> MANPYERGPNPTDALLEARSGPFSVSEERASRFGADGFGGGTIYYPRENNTYGAVAISPGYTGTQASVAWLGERIASHGFVVITIDTNTTLDQPDSRARQLNAALDYMINDASSAVRSRIDSSRLAVMGHSMGGGGTLRLASQRPDLKAAIPLTPWHLNKNWSSVRVPTLIIGADLDTIAPVLTHARPFYNSLPTSISKAYLELDGATHFAPNIPNKIIGKYSVAWLKRFVDNDTRYTQFLCPGPRDGLFGEVEEYRSTCPFAL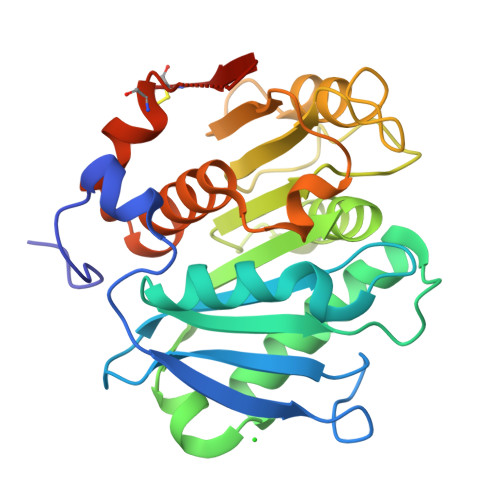E> MGGSHHHHHHGMASLAPGSSRVELFKRQSSKVPFEKDGKVTERVVHSFRLPALVNVDGVMVAIADARYETSFDNSLIDTVAKYSVDDGETWETQIAIKNSRASSVSRVVDPTVIVKGNKLYVLVGSYNSSRSYWTSHGDARDWDILLAVGEVTKSTAGGKITASIKWGSPVSLKEFFPAEMEGMHTNQFLGGAGVAIVASNGNLVYPVQVTNKKKQVFSKIFYSEDEGKTWKFGKGRSAFGCSEPVALEWEGKLIINTRVDYRRRLVYESSDMGNTWLEAVGTLSRVWGPSPK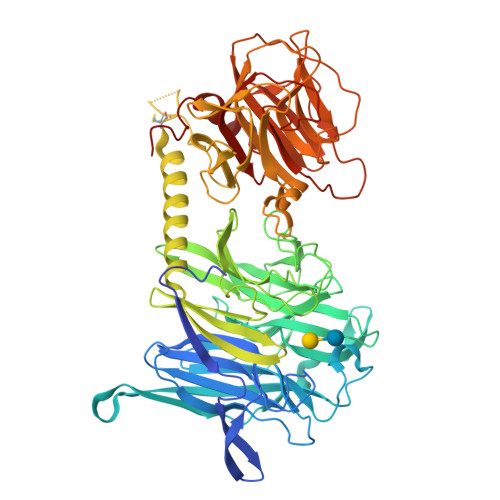SNQPGSQSSFTAVTIEGMRVMLFTHPLNFKGRWLRDRLNLWLTDNQRIYNVGQVSIGDENSAHSSVLYKDDKLYCLHEINSNEVYSLVFARLVGELRIIKSVLQSWKNWDSHLSSICTPADPAASSSERGCGPAVTTVGLVGFLSHSATKTEWEDAYRCVNASTANAERVPNGLKFAGVGGGALWPVSQQGQNQRYHFANHAFTLVASVTIHEVPKGASPLLGASLDSSGGKKLLGLSYDKRHQWQPIYGSTPVTPTGSWEMGKRYHVVLTMANKIGSVYIDGEPLEGSGQTVVPDERTPDISHFYVGGYKRSGMPTDSRVTVNNVLLYNRQLNAEEIRTLFLSQDLIGTEAHMD> AECSVDIQGNDQMQFNTNAITVDKSCKQFTVNL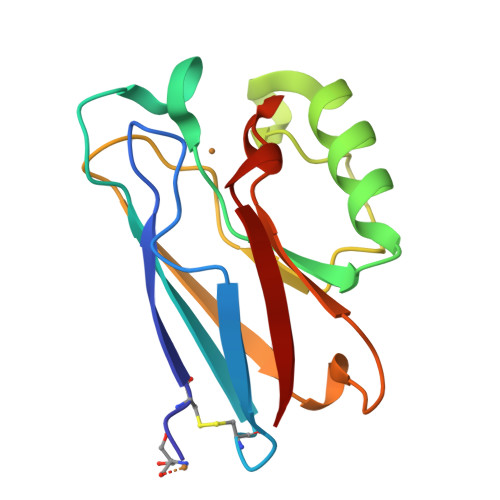SHPGNLPKNVMGHNWVLSTAADMQGVVTDGMASGLDKDYLKPDDSRVIAHTKLIGSGEKDSVTFDVSKLKEGEQYMFFDTFPGHSALMKGTLTLK Among the few candidates, the alcohol dehydrogenase from Thauera aromatica (ThaADH) stands out with a high activity for the reduction of the cyclic α‐diketone 1,2‐cyclohexanedione to the corresponding α‐hydroxy ketone. The results obtained confirm the previously observed preference of ThaADH for cyclic carbonyl compounds over aromatic and linear aliphatic compounds. This preference is in line with the physiological function of the enzyme, i. e. the oxidation of the cyclic 6‐hydroxycyclohex‐1‐ene‐1‐carboxyl‐CoA within the benzoyl‐CoA metabolism. The overall structural fold of ThaADH was consistent with those of many other MDR−ADHs, i. e. contains the typical C‐terminal coenzyme binding domain and N‐terminal catalytic domain. ThaADH shares with many ADHs of the MDR family the presence of two zinc atoms per monomer.

In this context, we determined the X‐ray crystallographic structure of the wild type (WT) ThaADH in complex with NADH, refined to a resolution of 2.60 Å, as well as of the double mutant K319A/K320A without cofactor, refined to 1.80 Å. Second, the K319A/K320A double mutant, which was obtained with one molecule in the asu and was refined to 1.80 Å, but no density for the cofactor was observed in the omit maps. Four cysteine residues coordinate the structural zinc in the catalytic domain: C94, C97, C100 and C108. Resolving the structure of WT ThaADH and a double mutant and comparing this to related well‐studied MDR−ADHs with preference for phenyl substituted and linear aliphatic substrates, gave novel insights into the underlying structure‐function relationships, which in the future might enable the rational design of MDR−ADHs towards acceptance of a wider range of diketones and their corresponding alcohols.

> MSSNPHRWMMTSPGAPMVRAEFEIGELSADQVVVAVAGCGVCHTDLGYYYDSVRTNHALPLALGHEISGRVVQAGANAAQWLGRAVIVPAVMPCGTCELCTSGHGTICRDQVMPGNDIQGGFASHVVVPARGLCPVDEARLAAAGLQLADVSVVADAVTTPYQAVLQAGVEPGDVAVVIGVGGVGGYAVQIANAFGASVVAIDVDPAKLEMMSKHGAALTLNAREISGRDLKKAIEAHAKANGLRLTRWKIFECSGTGAGQTSAYGLLTHGATLAVVGFTMDKVEVRLSNLMAFHARALGNWGCLPEYYPAALDLVLDAAIDLASFIERHPLDQIGEVFAAAHAHKLTRRAILTP> GSHMEEKEILWNEAKAFIAACYQELGKAAEVKDRLADIKSEIDLTGSYVHTKEELEHGAKMAWRNSNRCIGRLFWNSLNVIDRRDVRTKEEVRDALFHHIETATNNGKIRPTITIFPPEEKGEKQVEIWNHQLIRYAGYESDGERIGDPASCSLTAACEELGWRGERTDFDLLPLIFRMKGDEQPVWYELPRSLVIEVPITHPDIEAFSDLELKWYGVPIVSDMKLEVGGIHYNAAPFNGWYMGTEIGARNLADEKRYDKLKKVASVIGIAADYNTDLWKDQALVELNKAVLHSYKKQGVSIVDHHTAASQFKRFEEQAEEAGRKLTGDWTWLIPPISPAATHIFHRSYDNSIVKPNYF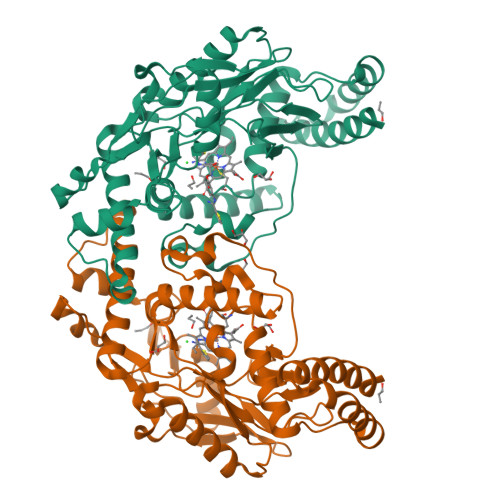YQDKPYE> MQSSTSTDQHVLHHMDPHRFTSQIPTATSSQLRRRNSTNQGLTDMINKSIARNTISGTGIPTGGINKNKRTRSTVAGGTNGTALALNDKSNSRNSVSRLSINQLGSLQQHLSNRDPRPLRDKNFQSAIQEEIYDYLKKNKFDIETNHPISIKFLKQPTQKGFIIIFKWLYLRLDPGYGFTKSIENEIYQILKNLRYPFLESINKSQISAVGGSNWHKFLGMLHWMVRTNIKLDMCLNKVDRSLINQNTQEITILSQPLKTLDEQDQRQERYELMVEKLLIDYFTESYKSFLKLEDNYEPSMQELKLGFEKFVHIINTDIANLQTQNDNLYEKYQEVMKISQKIKTTREKWKALKSDSNKYENYVNAMKQKSQEWPGKLEKMKSECELKEEEIKALQSNISELHKILRKKGISTEQFELQNQEREKLTRELDKINIQSDKLTSSIKSRKLEAEGIFKSLLDTLRQYDSSIQNLTRSRSQLGHNVNDSSLKINISENLLDRDFHEGISYEQLFPKGSGINESIKKSILKLNDEIQERIKTIEKDNITLEKDIKNLKHDINEKTQINEKLELELSEANSKFELSKQENERLLVAQRIEIEKMEKKINDSNLLMKTKISDAEELVTSTELKLEELKVDLNRKRYKLHQQVIHVIDITSKFKINIQSSLENSENELGNVIEELRNLEFETEHNVTN;> MSRNQDVFPILDLQELVICLQSCDFALATQENISRPTSDYMVTLYKQIIENFMGISVESLLNSSNQETGDGHLQEENENIYLDTLNVLVLNKICFKFFENIGVQDFNMTDLYKPEAQRTQRLLSAVVNYARFREERMFDCNSFILQMESLLGQLRSKFDDYNLIQQQLKQYEDVDGDNIPDEQELQKLEEQNKELEIQLKKLTKIQETLSIDYNDYKISKQSIFKDLEALSFQIVELESNRDKLIKISNTDMEELSEGIKELNDLLIQRKKTLDDLTAQQKNLQDTVTTFETIISELYDVLRIISSEVQESNRTETELVGLKQNLINNKLKLMNVLETGIMYKLEILQEQLDLQLKNLEKLSQDTKEESRLNDTKLMDLQIKYENEIKPKIDKTDIFIQEELISGKINKLNDEIKQLQKDFEVEVKEIEIEYSLLSGHINKYMNEMLEYMQ;> MSEDKAKLGTTRSATEYRLSIGSAPTSRRSSMGESSSLMKFADQEGLTSSVGEYNENTIQQLLLPKIRELSDSIITLDSNFTRLNFIHESLADLNESLGSLLYGIMSNSWCVEFSQAPHDIQDDLIAIKQLKSLEDEKNNLVMELSNMERGIKRKKDEQGENDLAKASQNKQFNQPLFPSSQVRKYRSYDNRDKRKPSKIGNNLQVENEEDYEDDTSSEASFVLNPTNIGMSKSSQGHVTKTTRLNNNTNSKLRRKSILHTIRNSIASGADLPIENDNVVNLGDLHPNNRISLGSGAARVVNGPVTKNRNSMFSGRAERKPTESRHSVAKKTEKKINTRPPFR;> MSEQSQLDDSTIDKLIPQIFNEMRSNLNNTTNKFPKSTGGGASDNISANSNSIRSFNSITTQSLLKESESLDKITAMIKNVTAALKNNLPVYVNQVHEVCKSTNSILDSWINIHSQAGYIHKLMSDQTYLKLINDRLHNENVNTNDEDGSTLHNVIALKKKEILDLRQKLENRKGEKDAAPAKPPNQGLNPRYGVQSGRRPVPSAGISNNGRVRKTHVPASKRPSGIPRVTNRWTKPTASSSRKMFR;> MDSIDEQIAIKRKELQSLQKITSLTDGLKIQLTELNEQIKEMGMNADSVAQLMNNWDSIINNISQASLGLLQYAEGDYEIGPWKDSKKKESEQSNETGLEAQENDKNDEDNDEDEDLVPLPETMVRIRVDGNE;> MMASTSNDEEKLISTTDKYFIEQRNIVLQEINETMNSILNGLNGLNISLESSIAVGREFQSVSDLWKTLYDGLESLSDEAPIDEQPTLSQSKTK;> MENPHEQVQANILSRIIGNVKRLNESVAILNQELVTINNRNKNLEIMGAICDNYHSSVQFNLEATNNKKPPL;> MEHNLSPLQQEVLDKYKQLSLDLKALDETIKELNYSQHRQQHSQQETVSPDEILQEMRDIEVKIGLVGTLLKGSVYSLILQRKQEQESLGSNSK;> MGESLDRCIDDINRAVDSMSTLYFKPPGIFHNAILQGASNKASIRKDITRLIKDCNHDEAYLLFKVNPEKQSVSRRDGKEGVFDYVIKRDTDMKRNRRLGRPGEKPIIHVPKEVYLNKDRLDLNNKRRRTATTSGGGLNGFIFDTDLIGSSVISNSSSGTFKALSAVFKDDPQIQRLLYALENGSVLMEEESNNQRRKTIFVEDFPTDLILKVMAEVTDLWPLTEFKQDYDQLYHNYEQLSSKLRFIKKEVLLQDDRLKTMSQYHPSSSHDVAKIIRKEKDEIRRLEMEIANLQE;> MDSASKEETLEKLDQEITVNLQKIDSNLSFCFHKITQDIIPHVATYSEICERIMDSTEWLGTMFQETGLVNLQANAAAPVGNAPVKSLVSNNVGIFPTSAEEASRQSQTDNGPNEADSAVHVNRDVHSMFNNDSIDDFHTANITSTGQILKLPDSSDEDTGSEAVPSREQTDLTGEGHGGADDEQDESTIQRQSRKRKISLLLQQQYGSSSSMVPSPIVPNKMRKQLAHEEHINNDGDNDDENSNNIESSPLKQGHHHPKGQADDNNEGPDEEESTKEVPKPGTIIHFSTNR;> MNANKQRQYNQLAHELRELQTNLQETTKQLDIMSKQCNENLVGQLGKVHGSWLIGSYIYYMEQMLGKTQ;> MTDALEQSVLALEGTVSVLKDSVESLKCANEPSTNLASTMLQTKRVFRLVPEYDVERSKLDLIEEVEPLVRTLGDKLRKSMGRMQRELDTLQQTYELNDLRLKKNISMDDDDALNSPDMGQEYEGRDADDVVMMASSTNEELEELKKLKEKKKQLENKLEILKQK

Kinetochores couple chromosomes to the mitotic spindle to segregate the genome during cell division. Knl1c functions in the spindle-assembly checkpoint (SAC), whereas Ndc80c, a heterotetramer of Ndc80, Nuf2, Spc24 and Spc25, is the major microtubule-binding component of KMN. Many fungi, including S. cerevisiae, utilize the ten-subunit Dam1 complex (Dam1c), which self-assembles into a large ring around microtubules, whereas most metazoans contain the Ska complex. Here we describe the cryo-electron microscopy structure of the budding yeast outer kinetochore Ndc80 and Dam1 ring complexes assembled onto microtubules.

Cryo-EM density was not visible for the Spc24:Spc25 subunits of Ndc80c. The coiled-coils of Ndc80c emanate from the calponin homology (CH) domains of the Ndc80 and Nuf2 subunits (Ndc80CH and Nuf2CH) at the surface of the microtubule to fold across the outer surface of the Dam1cRing. Our structure is consistent with previous cross-linking mass spectrometry and insertion mutagenesis experiments indicating that the central segment of the Ndc80:Nuf2 coiled-coils proximal to the conserved Ndc80 loop directly interacts with the Spc34:Spc19 C-termini. Following focused classification and flexible refinement, a distinct interruption in the coiled-coil became apparent. The flexible hinge between Ndc80cCH and Ndc80Loop permits Ndc80 complexes to fold as hooks across the Dam1cRing, explaining how the coiled-coils of Ndc80:Nuf2 dock in a parallel configuration across Spc19:Spc34 despite adherence of the Ndc80cCH to the pseudo-helical symmetry of the microtubule. Mutation of a series of four conserved interfacial residues on Ndc80 (Ndc80CC-mut1&2) did not impair viability, consistent with in vitro observations that disruption of this interface by phosphorylation of Spc34 at Thr199 exerts a minor reduction in outer kinetochore – microtubule rupture forces. In contrast, the Ndc80CC-mut2 (Spc19:Spc34-Ndc80:Nuf2 coiled-coil contact-2) essentially had no effect on rupture strength when combined with Dam1c. Our molecular models therefore account for two EC-sensitive contacts: the Dam1C-ter-Ndc80cCH and the Spc34-Ndc80:Nuf2CC interfaces. At both, residues phosphorylated in EC would cause electrostatic and steric repulsion, explaining how EC-mediated phosphorylation suppresses kinetochoreDam1c:Ndc80c assembly.> GPGSMTTRSARVIIASTRASSGEYEDRCGPIITEWLAQQGFSSAQPEVVADGSPVGEALRKAIDDDVDVILTSGGTGIAPTDSTPDQTVAVVDYLIPGLAEAIRQSGLPKVPTSVLSRGVCGVAGQTLIVNLPGSPGGVRDGLGVLAGVLDHALDQLAGKDHP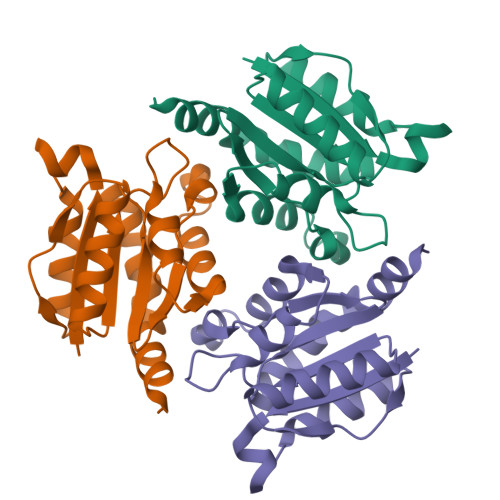R> GYVPQSVDNPNNLGDLPE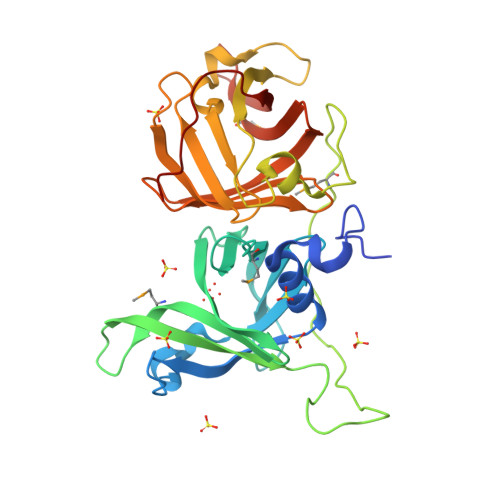YLRSVGIRQDEGLSEKDWAGTRVYDRNGNDLTDENQNLLHAIKFDATTSFYEFFDKETGESTGDEGTFFMTAGITDVSRLVIISETKNYQGVYPLRTLYQDTFTYRQMGKDKNGNDIEVFVENKATSGPVYGRPQPYPNNRPRTLEFTNGRRAMTEQTGQIDVNRQGDEIIGKTSFDGTPQLLWNGTKVVDKDGNDVTSANQNFISLAKFDQDSSKYEFFNLQTGETRGDYGYFKVGNQNKFRAHVSIGTNRYGAVLELTELNDNRFTYTRMGKDNEGNDIQVYVEHEPYQGTFNPEFTF The Eph (erythropoietin-producing hepatocyte) transmembrane receptor tyrosine kinase superfamily, with its first member identified30 years ago, contains 14 members in mammals and is the largest among all receptor tyrosine kinase families. However, the cytoplasmic portion of all 14 Eph receptors are highly similar, each containing a membrane-juxtaposing kinase domain, a protein-binding SAM domain immediately followed by a short carboxyl tail PDZ domain-binding motif (PBM). In this study, we performed systematic biochemical and structural studies of the bindings of three SAM domains, two from previously identified Eph-binding proteins (SHIP2 and Odin) and one from a new Eph-binding protein discovered in this study (SAMD5), to the SAM domains from every Eph receptor. Our study reveals that the Eph SAM domains have exquisitely specific target SAM domain-binding properties, although their overall SAM-SAM heterodimer formation modes are very similar.

The results showed that, similar to SHIP2 SAM, Odin SAM1 only selectively bound to the SAM domains from EphA1/EphA2/EphA6. To elucidate the molecular mechanism governing the specificity of the bindings of SHIP2 SAM and Odin SAM1 to Eph receptors, we determined the crystal structure of the SHIP2 SAM-EphA2 SAM complex and the Odin SAM1-EphA6 SAM complex at the 1.5 Å and 1.3 Å resolutions, respectively. The crystals diffracting at very high resolutions of both complexes were facilitated by fusing the Eph SAM domain to the C-terminal tail of the SHIP2 SAM or Odin SAM1 with a flexible linker (14 residues ‘SSGENLYFQSGSSG’ for the SHIP2 SAM-EphA2 SAM complex; 17 residues ‘PSGSSGENLYFQSGSSG’ for the Odin SAM1-EphA6 SAM complex). The covalent linkage did not appear to affect the overall structure of the complexes, as the linkers in both complexes are sufficiently long and flexible. The two complex structures adopt an essentially identical End-Helix/Mid-Loop binding mode, in which positively charged residues from the N-terminal end of α5 (End-Helix) of EphA2/EphA6 bind to negatively charged residues from the loop connecting α2-α4 (Mid-Loop) from SHIP2/Odin, forming the well-known tail-to-head SAM domain heterodimer. A noticeable feature in both complexes is that the backbone methylene of a Gly residue at the beginning of α5 from Eph SAM (Gly954A2/Gly1104A6) is in close contact with an aromatic residue from SHIP2/Odin SAM (Trp1221SHIP2/Phe738Odin). As such, replacing Gly at the beginning of α5 of Eph SAM with any other amino acid residues will introduce steric hindrance in preventing their binding to SHIP2/Odin SAM. The very high-resolution crystal structures of the two complexes also allowed us to identify a unique interaction feature that is critical for the exquisite specific interaction between the EphA2/A6 SAM domain and SHIP2/Odin SAM domains. Finally, EphA6 SAM could bind to both SAMD5 and SHIP2/Odin SAM domains, since it satisfies the binding criteria of both types.

>EGDIHMHHHHHHSSGLEVLFQGPGSISGSRTLEQSVGEWLESIGLQQYESKLLLNGFDDVRFLGSNVMEEQDLREIGISDPQHRRKLLQAARSLPKVKPSGSSGENLYFQSGSSGPEYPLFVTVGDWLDSIKMGQYKSNFMAAGFTTFDLISRMSIDDIRRIGVILIGHQRRIVSSIQTLRLHMMHIQEKGFHV[2x]>MRFIHALLLAGIAHSAYASEKLTFKTDLEKLEREKAAQIGVAIVDPQGEIVAGHRMAQRFAMCSTFKFPLAALVFERIDSGTERGDRKLSYGPDMIVEWSPATERFLASGHMTVLEAAQAAVQLSDNGATNLLLREIGGPAAMTQYF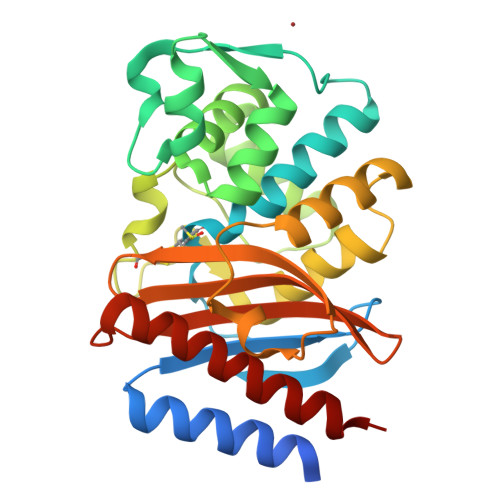RKIGDSVSRLDRKEPEMSDNTPGDLRDTTTPIAMARTVAKVLYGGALTSTSTHTIERWLIGNQTGDATLRAGFPKDWVVGEKTGTCANGGRNDIGFFKAQERDYAVAVYTTAPKLSAVERDELVASVGQVITQLILSTDK[2x]>MDFSRNLYDIGEQLDSEDLASLKFLSLDYIPQRKQEPIKDALMLFQRLQEKRMLEESNLSFLKELLFRINRLDLLITYLNTRKEEMERELQTPGRAQISAYRVMLYQISEEVSRSELRSFKGGLQEEISKCKLDDDMNLLDIFIEMEKRVILGEGKLDILKRVCAQINKSLLKIINDYEEFSKER[4x];>GSHMSAEVIHQVEEALDTDEKEMLLFLCRDVAIDVVPPNVRDLLDILRERGKLSVGDLAELLYRVRRFDL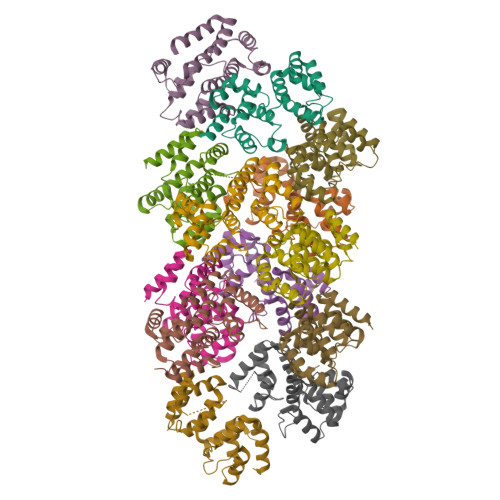LKRILKMDRKAVETHLLRNPHLVSDYRVLMAEIGEDLDKSDVSSLIFLMKDYMGRGKISKEKSFLDLVVELEKLNLVAPDQLDLLEKCLKNIHRIDLKTKIQKYKQSVQGAGTS[9x]>MAHH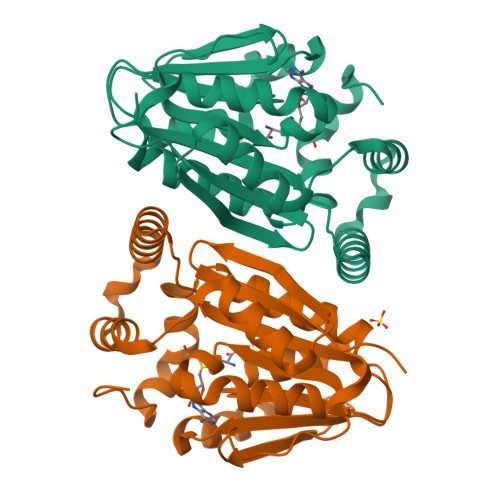HHHHVDDDDKMSHRDTLFSAPIARLGDWTFDERVAEVFPDMIQRSVPGYSNIISMIGMLAERFVQPGTQVYDLGCSLGAATLSVRRNIHHDNCKIIAIDNSPAMIERCRRHIDAYKAPTPVDVIEGDIRDIAIENASMVVLNFTLQFLEPSERQALLDKIYQGLNPGGALVLSEKFSFEDAKVGELLFNMHHDFKRANGYSELEISQKRSMLENVMLTDSVETHKARLHKAGFEHSELWFQCFNFGSLVALKAEDAA[2x]>[6x]MKFSKEQFDYSLYLVTDSGMIPEGKTLYGQVEAGLQNGVTLVQIREKDADTKFFIEEALQIKELCHAHNVPLIINDRIDVAMAIGADGIHVGQDDMPIPMIRKLVGPDMVIGWSVGFPEEVDELSKMGPDMVDYIGVGTLFPTLTKKNPKKAPMGTAGAIRVLDALERNNAHWCRTVGIGGLHPDNIERVLYQCVSSNGKRSLDGICVVSDIIASLDAAKSTKILRGLIDKTDYKFVNIGLSTKNSLTTTDEIQSIISNTLKARPLVQHITNKVHQNFGANVTLALGSSPIMSEIQSEVNDLAAIPHATLLLNTGSVAPPEMLKAAIRAYNDVKRPIVFDPVGYSATETRLLLNNKLLTFGQFSCIKGNSSEILGLAELNKERMKGVDASSGISNELLIQATKIVAFKYKTVAVCTGEFDFI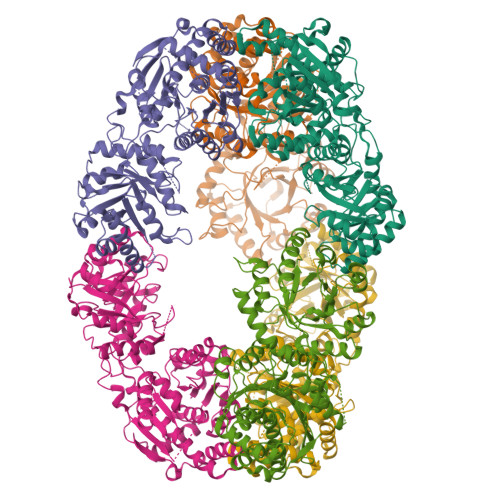ADGTIEGKYSLSKGTNGTSVEDIPCVAVEAGPIEIMGDITASGCSLGSTIACMIGGQPSEGNLFHAVVAGVMLYKAAGKIASEKCNGSGSFQVELIDALYRLTRENTPVTWAPKLTHT> NAEFVTQLACKYWAPHIKKKSPFDIKVIEDIYEKEIVKSRFAIRKIMLLEFSQYLENYLWMNYSPEVSSKAYLMSICCMVNEKFRENVPAWEIFKKKPDHFPFFFKHILKAALAETDGEFSLHEQTVLLLFLDHCFNSLEVDLIRSQVQQLISLPMWMGLQLARLELELKKTPKLRKFWNLIKKNDEKMDPEAREQAYQERRFLSQLIQKFISVLKSVPLSEPVTMDKVHYCERFIELMIDLEALLPTRRWFNTILDDSHLLVHCYLSNLVRREEDGHLFSQLLDMLKFYTGFEINDQTGNALTENEMTTIHYDRITSLQRAAFAHFPELYDFALSNVAEVDTRESLVKFFGPLSSNTLHQVASYLCLLPTLPKNEDTTFDKEFLLELLVSRHERRISQIQQLNQMPLYPTEKIIWDENIVPTEYYSGEGCLALPKLNLQFLTLHDYLLRNFNLFRLESTYEIRQDIEDSVSRMKPWQSEYGGVVFGGWARMAQPIVAFTVVEVAKPNIGENWPTRVRADVTINLNVRDHIKDEWEGLRKHDVCFLITVRPTKPYGTKFDRRRPFIEQVGLVYVRGCEIQGMLDDKGRVIEDGPEPRPNLRGESRTFRVFLDPNQYQQDMTNTIQNGAEDVYETFNIIMRRKPKENNFKAVLETIRNLMNTDCVVPDWLHDIILGYGDPSSAHYSKMPNQIATLDFNDTFLSIEHLKASFPGHNVKVTVEDPALQIPPFRITFPVRSGKGKKRKDADVEDEDTEEAKTLIVEPHVIPNRGPYPYNQPKRNTIQFTHTQIEAIRAGMQPGLTMVVGPPGTGKTDVAVQIISNIYHNFPEQRTLIVTHSNQALNQLFEKIMALDIDERHLLRLGHGEEELETEKDFSRYGRVNYVLARRIELLEEVKRLQKSLGVPGDASYTCETAGYFFLYQVMSRWEEYISKVKNKGSTLPDVTEVSTFFPFHEYFANAPQPIFKGRSYEEDMEIAEGCFRHIKKIFTQLEEFRASELLRSGLDRSKYLLVKEAKIIAMTCTHAALKRHDLVKLGFKYDNILMEEAAQILEIETFIPLLLQNPQDGFSRLKRWIMIGDHHQLPPVIKNMAFQKYSNMEQSLFTRFVRVGVPTVDLDAQGRARASLCNLYNWRYKNLGNLPHVQLLPEFSTANAGLLYDFQLINVEDFQGVGESEPNPYFYQNLGEAEYVVALFMYMCLLGYPADKISILTTYNGQKHLIRDIINRRCGNNPLIGRPNKVTTVDRFQGQQNDYILLSLVRTRAVGHLRDVRRLVVAMSRARLGLYIFARVSLFQNCFELTPAFSQLTARPLHLHIIPTEPFPTTRKNGERPSHEVQIIKNMPQMANFVYNMYMHLIQTTHHYHQTLLQLPPAMVEEGEEVQNQETELETEEEAM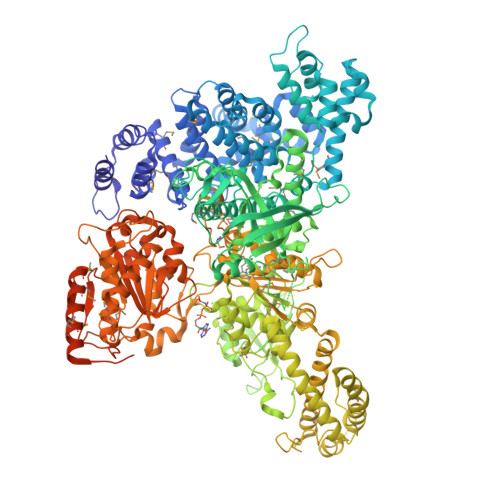TVQADIIPSPTDTSCRQETPAFQTDTTPSETGATSTPEAIPALSETTPTVVGAVSAPAEANTPQDATSAPEETKHHHHHHHH>GGTTAGGGTTCTTGAACCCTTGGGTTACTTGTAACC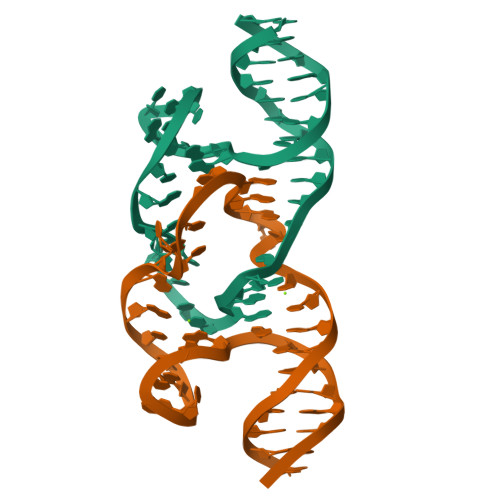CTAACC[2x]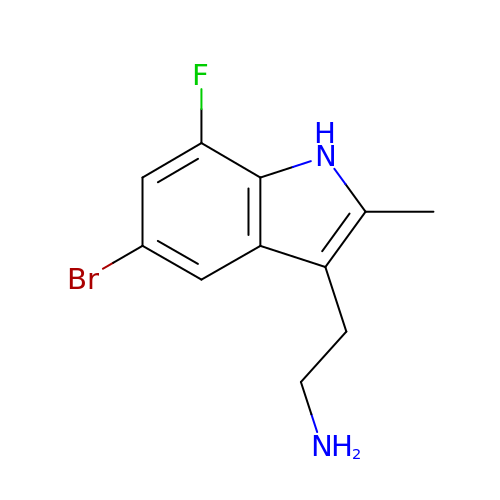2-(5-bromanyl-7-fluoranyl-2-methyl-1H-indol-3-yl)ethanamine | C11 H12 Br F N2 | ZXTLEYKPUYPREL-UHFFFAOYSA-N>MSRVQMDTEEVREFVGHLERFKELLREEVNSLSNHFHNLESW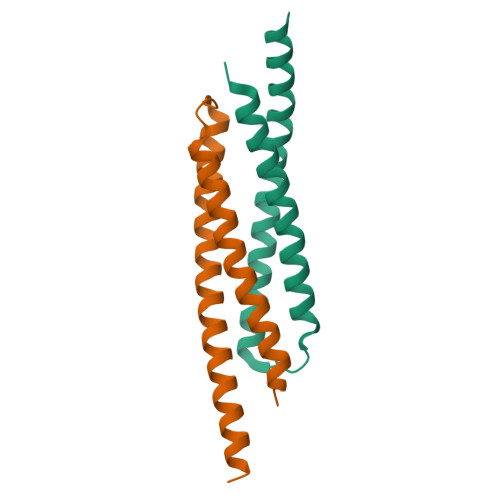RDARRDKFSEVLDNLKSTFNEFDEAAQEQIAWLKERIRVLEEDYLEHHHHHH[2x]> XSTVHEILSKLS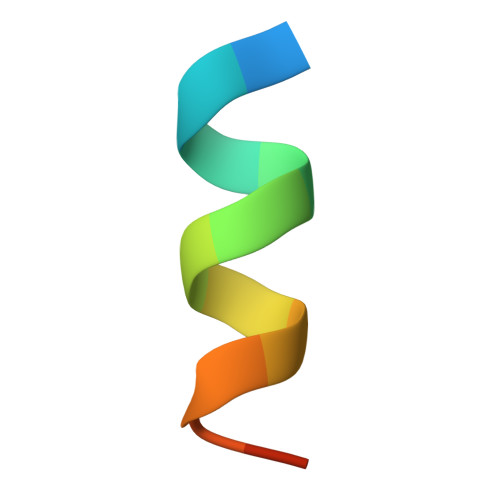LE>MAQERKVALVTGASRGIGAAIAQQLIQDGYFVVGTATSESGAQKLTDSFGEQGAGLALDVRNLDEIEAVVSHIEQNYGPVLVLVNNAGITKDNLLLRMSEDDWDDILNIHLKAVYRLSKRVLKGMTKARFGRIINISSVVAHFANPGQANYSAAKAGIEAFSRSLAKEMGSRQITVNSVAPGFIATEMTDALSEDIRKKMSDQVALNRLGEPQDIANAVSFLASDK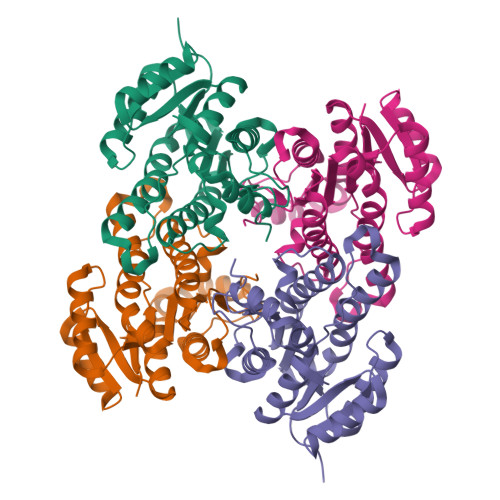AGYITGTVLHVNGGLYMA[2x]> GGSGRPEIWIAQEL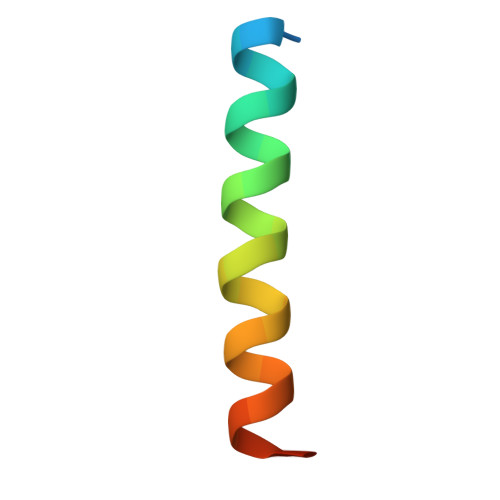RRIGDEFNAYYARRV{4-[(6-chloroquinoxalin-2-yl)oxy]phenyl}acetic acid | C16 H11 Cl N2 O3 | 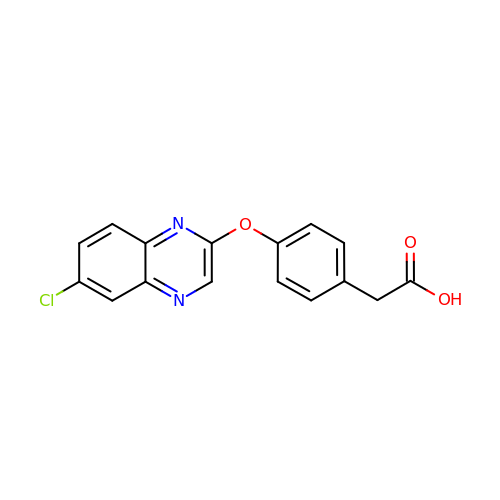SPHMJKAQMWKCCP-UHFFFAOYSA-N> TARSKVGGSGDQTWVQCDACLKWRKLPDGMDQLPEKWYCSNNPDPQFRNCEVPEE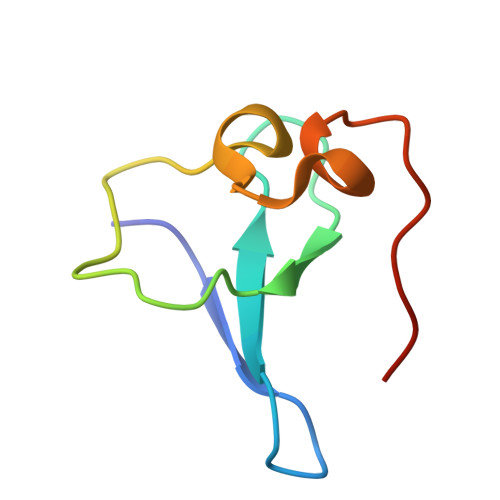PEDE Following oxidation of the α-hydroxyl group in GGE by a Cα-dehydrogenase, stereospecific glutathione (GSH)-dependent cleavage of the β-ether linkage in β-(3′-methoxyphenoxy)-γ-hydroxypropiovanillone (MPHPV) is catalyzed by the glutathione S-transferase (GST) enzymes LigE and LigF, forming β-glutathionyl-γ-hydroxypropiovanillone (GS-HPV) and guaiacol. LigE catalyzes stereospecific cleavage of (βR)-MPHPV to (βS)-GS-HPV, whereas LigF catalyzes the cleavage of (βS)-MPHPV to (βR)-GS-HPV. Consistent with their classification as GST enzymes, LigE and LigF each adopt the canonical GST domain fold with an N-terminal thioredoxin domain (residues 1–82 and 1–76, respectively) and a C-terminal α-helical domain (residues 93–255 and 93–242, respectively) connected by a short linker (residues 83–92 and 77–92, respectively). Biochemical and small angle x-ray scattering data suggest that both LigE and LigF exist as dimers in solution, and these dimers, related by 2-fold symmetry, can be seen in the respective crystal structures.

Attempts to solve the structure of full-length wild-type LigE (282 residues) and LigF (254 residues) were unsuccessful, but C-terminal truncation constructs of both proteins were generated, successfully crystallized, and used for structural analysis. LigEΔ255 and the LigEΔ255-GSH complex crystallized in the space group C2 with four molecules in the asymmetric unit with electron density for the bound GSH molecule. In the LigE dimer, helix α4 of one monomer is interdigitated between α4 and α7 of the other monomer, and the entire dimer interface is contained within the α-helical domain. The dimer is anchored by a hydrophobic lock-and-key motif in which Phe-101 of each monomer is in a hydrophobic pocket formed in the second monomer. This motif is seen in several GST classes, including Alpha, Mu, and Phi, which display the more typical four-helix bundle dimer mode rather than the elongated dimer of LigE. An extended loop between α5 and α6 in the C-terminal domain, which protrudes above the normal α3/α4 packing site, may be responsible for the alternate dimer formation in LigE. The C-terminal domains of both LigE and LigF are composed of six and eight α-helices, respectively. The loop between β1 and α1 is longer in LigE than in LigF and occupies the space between the thioredoxin domain and the α-helical domain, whereas in LigF, this loop is moved away from the domain interface toward the surface of the thioredoxin domain. Based on structural properties, LigE is most similar to the fungal GSTFuA class, suggesting that the enzymes in this class are present in both prokaryotes and fungi.

>[4x]MARNNTITLYDLQLESGCTISPYVWRTKYALKHKGFDIDIVPGGFTGILERTGGRSERVPVIVDDGEWVLDSWVIAEYLDEKYPDRPMLFEGPTQKNLMKFLDNWLWSTAVGPWFRCYILDYHDLSLPQDRDYVRWSREQWFLGGQRLEDVQAGREDRLPLVPPTLEPFRRILAETKWLGGDQPNFADYSALAVFLWTASVARTPPLTEDDPLRDWLDRGFDLFDGLGRHPGMNPLFGLKLREGDPEPFVRQTGPAGAGGQALNKGPQTTKMPPRVAEKAD> DYKDDDDKVPHDGNERSHRIARLAAVVSGIAGLLLCGIVPLLPVNQTTATIFWPQGSTADGNITQITAPL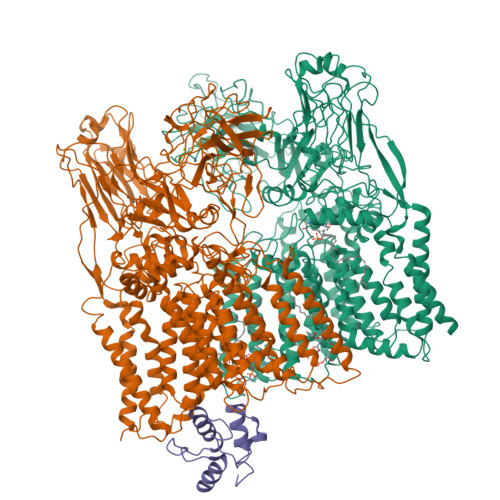VSGAPRALDISIPCSAIATLPANGGLVLSTLPAGGVDTGKAGLFVRANQDTVVVAFRDSVAAVAARSTIAAGGCSALHIWADTGGAGADFMGIPGGAGTLPPEKKPQVGGIFTDLKVGAQPGLSARVDIDTRFITTPGALKKAVMLLGVLAVLVAMVGLAALDRLSRGRTLRDWLTRYRPRVRVGFASRLADAAVIATLLLWHVIGATSSDDGYLLTVARVAPKAGYVANYYRYFGTTEAPFDWYTSVLAQLAAVSTAGVWMRLPATLAGIACWLIVSRFVLRRLGPGPGGLASNRVAVFTAGAVFLSAWLPFNNGLRPEPLIALGVLVTWVLVERSIALGRLAPAAVAIIVATLTATLAPQGLIALAPLLTGARAIAQRIRRRRATDGLLAPLAVLAAALSLITVVVFRDQTLATVAESARIKYKVGPTIAWYQDFLRYYFLTVESNVEGSMSRRFAVLVLLFCLFGVLFVLLRRGRVAGLASGPAWRLIGTTAVGLLLLTFTPTKWAVQFGAFAGLAGVLGAVTAFTFARIGLHSRRNLTLYVTALLFVLAWATSGINGWFYVGNYGVPWYDIQPVIASHPVTSMFLTLSILTGLLAAWYHFRMDYAGHTEVKDNRRNRILASTPLLVVAVIMVAGEVGSMAKAAVFRYPLYTTAKANLTALSTGLSSCAMADDVLAEPDPNAGMLQPVPGQAFGPDGPLGGISPVGFKPEGVGEDLKSDPVVSKPGLVNSDASPNKPNAAITDSAGTAGGKGPVGINGSHAALPFGLDPARTPVMGSYGENNLAATATSAWYQLPPRSPDRPLVVVSAAGAIWSYKEDGDFIYGQSLKLQWGVTGPDGRIQPLGQVFPIDIGPQPAWRNLRFPLAWAPPEADVARIVAYDPNLSPEQWFAFTPPRVPVLESLQRLIGSATPVLMDIATAANFPCQRPFSEHLGIAELPQYRILPDHKQTAASSNLWQSSSTGGPFLFTQALLRTSTIATYLRGDWYRDWGSVEQYHRLVPADQAPDAVVEEGVITVPGWGRPGPIRALP;> MTQCASRRKSTPNRAILGAFASARGTRWVATIAGLIGFVLSVATPLLPVVQTTAMLDWPQRGQLGSVTAPLISLTPVDFTATVPCDVVRAMPPAGGVVLGTAPKQGKDANLQALFVVVSAQRVDVTDRNVVILSVPREQVTSPQCQRIEVTSTHAGTFANFVGLKDPSGAPLRSGFPDPNLRPQIVGVFTDLTGPAPPGLAVSATIDTRFSTRPTTLKLLAIIGAIVATVVALIALWRLDQLDGRGSIAQLLLRPFRPASSPGGMRRLIPASWRTFTLTDAVVIFGFLLWHVIGANSSDDGYILGMARVADHAGYMSNYFRWFGSPEDPFGWYYNLLALMTHVSDASLWMRLPDLAAGLVCWLLLSREVLPRLGPAVEASKPAYWAAAMVLLTAWMPFNNGLRPEGIIALGSLVTYVLIERSMRYSRLTPAALAVVTAAFTLGVQPTGLIAVAALVAGGRPMLRILVRRHRLVGTLPLVSPMLAAGTVILTVVFADQTLSTVLEATRVRAKIGPSQAWYTENLRYYYLILPTVDGSLSRRFGFLITALCLFTAVFIMLRRKRIPSVARGPAWRLMGVIFGTMFFLMFTPTKWVHHFGLFAAVGAAMAALTTVLVSPSVLRWSRNRMAFLAALFFLLALCWATTNGWWYVSSYGVPFNSAMPKIDGITVSTIFFALFAIAAGYAAWLHFAPRGAGEGRLIRALTTAPVPIVAGFMAAVFVASMVAGIVRQYPTYSNGWSNVRAFVGGCGLADDVLVEPDTNAGFMKPLDGDSGSWGPLGPLGGVNPVGFTPNGVPEHTVAEAIVMKPNQPGTDYDWDAPTKLTSPGINGSTVPLPYGLDPARVPLAGTYTTGAQQQSTLVSAWYLLPKPDDGHPLVVVTAAGKIAGNSVLHGYTPGQTVVLEYAMPGPGALVPAGRMVPDDLYGEQPKAWRNLRFARAKMPADAVAVRVVAEDLSLTPEDWIAVTPPRVPDLRSLQEYVGSTQPVLLDWAVGLAFPCQQPMLHANGIAEIPKFRITPDYSAKKLDTDTWEDGTNGGLLGITDLLLRAHVMATYLSRDWARDWGSLRKFDTLVDAPPAQLELGTATRSGLWSPGKIRIGPHLGGIKAFHHHHHHHHHH;> MAATQEEIIAGLAEIIEEVTGIEPSEVTPEKSFVDDLDIDSLSMVEIAVQTEDKYGVKIPDEDLAGLRTVGDVVAYIQKLEEENPEAAAALREKFAADQ>[4x]MSNRPVALVSDTRYYVGPDLARRFAEKGFDLVL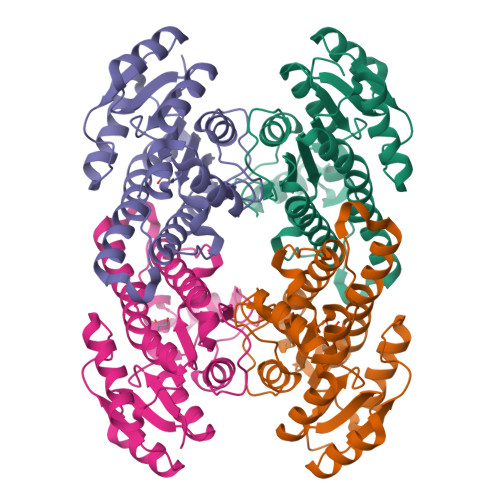GDPSPNLVSELESMGARIVPVTGHSDLSSPESAQAQADAALSAFGRLDSAVMFSGQIVTGRFVNSTIDQLRQVFVGCVEAPYNFMRAVVPVMTEREAGQILIITSASGARPTPGAPLYSSVRAAATMLVKNVADEVARTGVQVNAVGTNFMDFPAFLKASGANDPEVRAKIESQVPMRRLGTMEEFSAFCMAFLDGSSRFTTGQFVAYAGGWA>[2x]MGGHHHHHHGLEVLFQGPQEKDASSQGFLPHFQHFATQAIHVGQDPEQWTSRAVVPPISLSTTFKQGAPGQHSGFNYSRSGNPTRNCLEKAVAALDGAKYCLAFASGLAATVTITHLLKAGDQIICMDDVYGGTNLYFRQVASEFGLKISFVDCSKIKLLEAAITPETKLVWIETPTNPTQKVIDIEGCAHIVHKHGDIILVVDNTFMSPYFQRPLALGADISMYSATK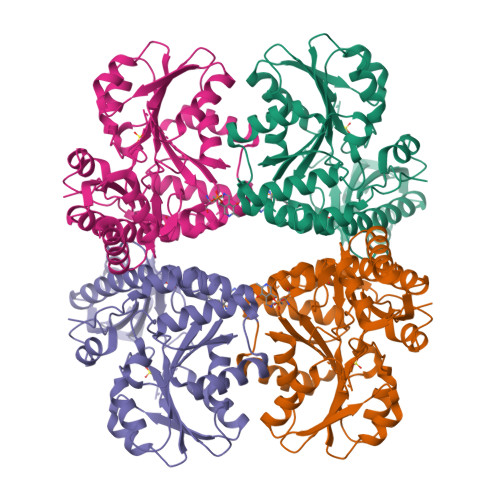YMNGHSDVVMGLVSVNCESLHNRLRFLQNSLGAVPSPIDCYLCNRGLKTLHVRMEKHFKNGMAVAQFLESNPWVEKVIYPGLPSHPQHELVKRQCTGCTGMVTFYIKGTLQHAEIFLKNLKLFTLAVSLGGFESLAELPAIMTHASVLKNDRDVLGISDTLIRLSVGLEDEEDLLEDLDQALKAAHPPSGIHS>HMSGRDISTAVVVTTISDGGFLDRLAPALRDAGARLIVIPDRNTGPALFAACERHRRLGLDVVCPSVAEQQDLLERLAVPDLIPYHSDNRRNVGYLMAWMEGFDVIVSMDDDNLPTTDDFVERHQVVCQGPRTQPVTASSDGWFNNCALLEVEPTEVFPRGFPFHARPAHAQARTSVCERPADVRINAGLWLGDPDVDAITRLAVRPNALAHSGGSVVLAEGTWCPVNSQNTAVHRDALPAYYFLRMGQPVDGVPMERFGDIFSGYFVQVCAQHLGHAVRFGDPVVEHPRNEHDLLDDLHKEVPAVRLLDDILDHLRDHPLEGGDYLETYESLSYALQEIAERVNGRAWSPDARAFLHRSAHLMRSWTGALRTVAGT[2x]

Members of glycosyltransferase family 75 (GT75) not only reversibly catalyze the autoglycosylation of a conserved arginine residue with specific NDP-sugars but also exhibit NDP-pyranose mutase activity that reversibly converts specific NDP-pyranose to NDP-furanose. MtdL from deep sea–derived Marinactinospora thermotolerans SCSIO 00652 has been discovered in the antibiotic A201A biosynthetic pathway, generating GDP-L-galactofuranose (L-Galf) from GDP-L-galactopyranose (L-Galp). The MtdL subunit is divided into three regions: the N-terminal region (residues 1–111), the core region (residues 112–291), and the C-terminal region (residues 292–376). The characteristic DXD motif (Asp109-Asp110-Asp111), together with conserved His287, coordinates a Mn2+ ion, which stabilizes the diphosphate of the nucleotide.

The initial structure of MtdL at 2.1-Å resolution was determined using single-wavelength anomalous diffraction phasing from cocrystals of selenomethionine (SeMet) derivative MtdL with GDP. However, the electron density of the GDP diphosphate moiety was poor. Then, the complex structure of MtdL bound to Mn2+ and GDP at 2.1-Å resolution was obtained by cocrystallizing MtdL containing 0.5 mM MnCl2 with GDP, which led to a clear electron density for both the GDP diphosphate moiety and the Mn2+ ion at the active site. Both SeMet-MtdL·GDP and MtdL·Mn2+·GDP structures contain two protein chains per asymmetric unit (ASU) that can be superimposed with root-mean-square deviations (RMSDs) of 0.079 A˚ and 0.081 A˚ over 308 and 353 Cα atoms, respectively. A tetramer as a dimer of dimers was suggested by PISA for crystal structures of both GDP·SeMet-MtdL belonging to space group C2 and GDP·Mn2+·MtdL belonging to space group C2221. Structural comparison of GDP-MtdL complexes in the absence and presence of Mn2+ indicated a major conformational change in loop A (residues 288–292), which follows the Mn2+ coordinating His287 on β15. This flexible loop, together with the diphosphate of GDP, showed poor electron density in the GDP bound structure without Mn2+.> HHHHHHSSGENLYFQGHMRPERLTVRNFLGLKNVDIEFQSGITVVEGPNGAGKSSLFEAISFALFGNGIRYPNSYDYVNRNAVDGTARLVFQFERGGKRYEIIREINALQRKHNAKLSEILENGKKAAIAAKPTSVKQEVEKILGIEHRTFIRTVFLPQ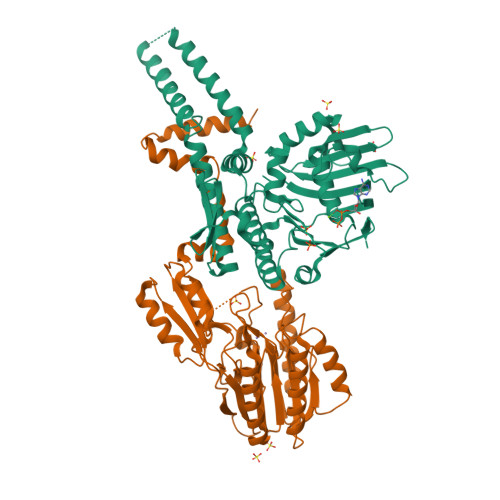GEIDKLLISPPSEITEIISDVFQSKETLEKLEKLLKEKMKKLENEISSGGAGGAGGSLEKKLKEMSDEYNNLDLLRKYLFDKSNFSRYFTGRVLEAVLKRTKAYLDILTNGRFDIDFDDEKGGFIIKDWGIERPARGLSGGERALISISLAMSLAEVASGRLDAFFIDEGFSSLCTENKEKIASVLKELERLNKVIVFITCDREFSEAFDRKLRITGGVVVNE;> MKILHTSDWHLGVTSWTSSRPVDRREELKKALDKVVEEAEKREVDLILLTGDLLHSRNNPSVVALHDLLDYLKRMMRTAPVVVLPGNQDWKGLKLFGNFVTSISSDITFVMSFEPVDVEAKRGQKVRILPFPYPDESEALRKNEGDFRFFLESRLNKLYEEALKKEDFAIFMGHFTVEGLAGYAGIEQGREIIINRALIPSVVDYAALGHIHSFREIQKQPLTIYPGSLIRIDFGEEADEKGAVFVELKRGEPPRYERIDASPLPLKTLYYKKIDTSALKSIRDSCRNFPGYVRVVYEEDSGILPDLMGEIDNLVKIERKSRREIEEVLRESPEEFKEELDKLDYFELFKEYLKKREENHEKLLKILDELLDEVKKSEA>MKTIIALSYIFCLVFAGGGGSPSRLEEELRRRLTEPQEMYAPHSIRIEGDVTLGGLFPVHAKGPSGVPCGDIKRENGIHRLEAMLYALDQINSDPNLLPNVTLGARILDTCSRDTYALEQSLTFVQALIQKDTSDVRCTNGEPPVFVKPEKVVGVIGASGSSVSIMVANILRLFQIPQISYASTAPELSDDRRYDFFSRVVPPDSFQAQAMVDIVKALGWNYVSTLASEGSYGEKGVESFTQISKEAGGLCIAQSVRIPQERKDRTIDFDRIIKQLLDTPNSRAVVIFANDEDIKQILAAAKRADQVGHFLWVGSDSWGSKINPLHQHEDIAEGAITIQPKRATVEGFDAYFTSRTLENNRRNVWFAEYWEENFNCKLTISGSKKEDTDRKCTGQERIGKDSNYEQEGKVQFVIDAVYAMAHALHHMNKDLCADYRGVCPEMEQAGGKKLLKYIRNVNFNGSAGTPVMFNKNGDAPGRYDIFQYQTTNTSNPGYRLIGQWTDELQLNIEDMQWGKGVR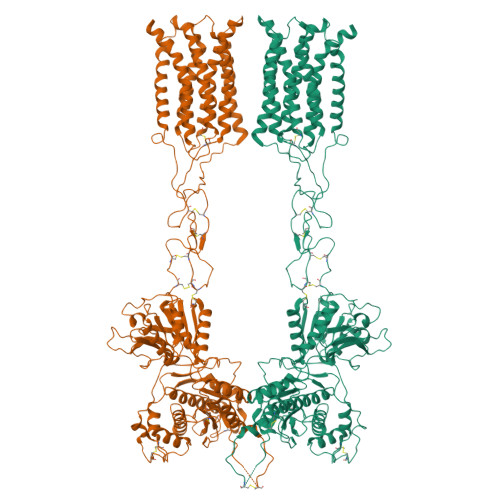EIPASVCTLPCKPGQRKKTQKGTPCCWTCEPCDGYQYQFDEMTCQHCPYDQRPNENRTGCQDIPIIKLEWHSPWAVIPVFLAMLGIIATIFVMATFIRYNDTPIVRASGRELSYVLLTGIFLCYIITFLMIAKPDVAVCSFRRVFLGLGMCISYAALLTKTYRIYRIFEQGKKSVTAPRLISPTSQLAITSSLISVQLLGVFIWFIVDPPNIIIDYDEHKTMNPEQARGVLKCDITDLQIICSLGYSILLMVTCTVYAFKTRGVPENFNEAKYIGFTMYTTCIVWLAFIPIFFGTAQSAEKLYIQTTTLTISMNLSASVALGMLYMPKVYIIIFHPELNVQKRKRSFKAVVTAATMSSRLSHKPSDRPNGEAKTELCENVDPNSPAAKKKYVSYNNLVI[2x]We identified C12orf29 (RLIG1) as an atypical ATP-grasp enzyme. Our biochemical and structural characterizations revealed this enzyme to be a 5’ to 3’ RNA ligase, structurally and functionally similar to phage T4 RNA ligase. Although the 5’ to 3’ RNA ligases contain the ATP-grasp fold, their catalytic mechanism is different from canonical members of this superfamily; they transfer an AMP moiety from ATP to the side-chain amino group of an active-site lysine to form a ligase-(lysyl-N)-AMP intermediate. To gain insight into the reaction mechanism of RLIG1, we solved crystal structures of WT (adenylated) and K73M Yasminevirus sp. GU-2018 (28) RLIG1 (YspRLIG1) in the presence of ATP.

In the WT structure, either AMP or ADP was modeled in the active site. In the YspRLIG1K73M structure, ATP was bound in the active site. Both structures were virtually identical; thus, we use the YspRLIG1K73M structure to describe the interactions related to catalysis. We superimposed the active sites of ADP-bound YspRLIG1WT with ATP-bound YspRLIG1K73M. In the ADP-bound YspRLIG1WT structure, the O5-Pα bond is rotated to flip the α-phosphate group toward the Nζ of Lys73. This situates the Nζ of Lys73 ~4Å away from the Pα of the ADP in an apical orientation to the β-phosphate group (Nζ-Pα-O3α angle = 144.4°). We believe this orientation more likely represents the conformation of the α-phosphate group during adenylation. Superposition of the YspRLIG1K73M and T4 Rnl1 active sites suggests that Asp75 (Motif I), Glu174 (Motif III), Glu240 (Motif IV), and Lys253 (Motif V) may be involved in Mg2+ binding. We modeled a Mg2+ ion in the electron density that is between 3.5 to 4 Å from these residues, which is a density that would be consistent with a Mg(H2O)62+ ion; however, we do not see the bound waters. Although YspRLIG1 shares the nucleotidyltransferase (NTase) domain of T4 Rnl1, it is missing the RNA binding domain.

>[6x]SMSDMNSESKSNTVSDKMCEVHDKISAILVCAHVKGTETEKAGRSGEKYLATNCLNPGLISAIQAGARVVPTAKTDGTCCRVFNGKIQKRRDIKPGREVPEGWIQTGSDEKSGHLIGFMDLEKGDKWHYDCHVKDPSSPSGLDINKVLCITTNKAGDALVYEEVNIADLNGHTVELMGPKFQSNPHGLKAHCLMRHGTVKLTDFPDLRDYVSVDGAEPLKENALADIRNWFLNSKQGPHLEGVVLHLDNGEMYKLHRHHLDLEWSAKSARPLDQIPL> GPGGSMKRLRPSDKFFELLGYKPHHVQLAIHRSTAKRRVACLGRQSGKSEAASVEAVFELFARPGSQGWIIAPTYDQAEIIFGRVVEKVERLAEVFPATEVQLQRRRLRLLVHHYDRPVNAPGAKRVATSEFRG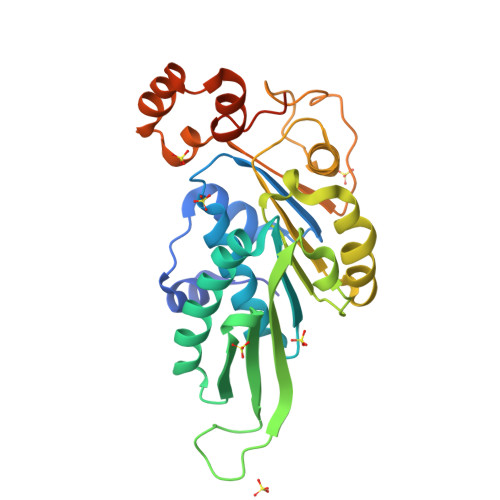KSADRPDNLAGATLDFVILDEAAMIPFSVWSEAIEPTLSVRDGWALIISTPKGLNWFYEFFLMGWRGGLKEGIPNSGINQTHPDFESFHAASWDVWPERREWYMERRLYIPDLEFRQEYGAEFVSHSGLEHHHHHHHHHH>[2x]SSDEEFKFLATEAKMLITAAERLAGTDPELQEMVALIKKELEQAERTFRNGDKSEAQRQLEFVLTAARAVMNVAAAANAAGTDPELIEMVLRILKQLKEAIRTFQNGDQEEAETQLRFVLRAAIAVAVVAAALVLAGTDPELQEMVKQILEELKQAIETFARGDKEKALTQLLFVAWAAHAVAMIAAAANLAGTDPRLQQQVKEILEKLKEAIETFQKGDEEQAFRQLAEVLAEAALVALRAALTN

To investigate the photophysics of special pairs independently of the complexities of native photosynthetic proteins, and as a first step toward creating synthetic photosystems for new energy conversion technologies, we designed C2-symmetric proteins that hold two chlorophyll molecules in closely juxtaposed arrangements. For Chl dimer protein scaffolds, we chose hyperstable C2-symmetric repeat protein dimers containing symmetric pockets with tunable sizes and geometries. In this dimeric repeat protein architecture, the hydrophobic core is independent of the small molecule-binding site, enabling full customization for binding with little impact on the overall protein structure. We describe de novo-designed proteins that hold Chl dimers in precisely defined, closely juxtaposed geometries.

SP2 was intended to assemble a ZnPPaM dimer with a conformation substantially different from that of native special pairs to investigate the effect of dimer geometry. The SP2 crystal structure was solved in both the apo state and the ZnPPaM-bound state to 2.4 and 2.5 Å resolution, respectively. The apo- and holo-state amino acid backbones both agree with the SP2 design model to within 1.4 Å r.m.s.d. Compared with the apo-state crystal structure, the SP2 binding cavity widens by ~1.6 Å in the presence of ZnPPaM; this expansion provides the extra volume needed for the ZnPPaM molecules to adopt their unexpected conformation.> HMSVNKVTCLVCRKGDN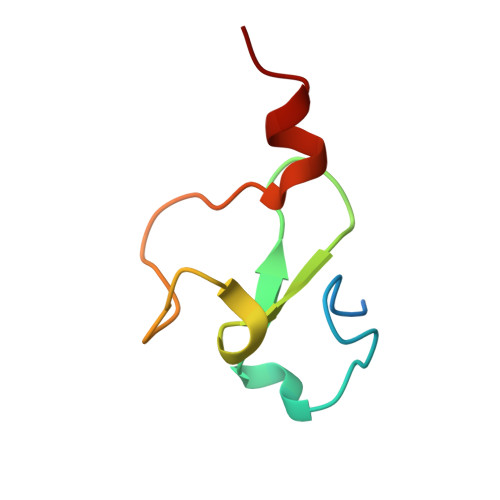DEFLLLCDGCDRGCHIYCHRPKMEAVPEGDWFCTVCLAQQV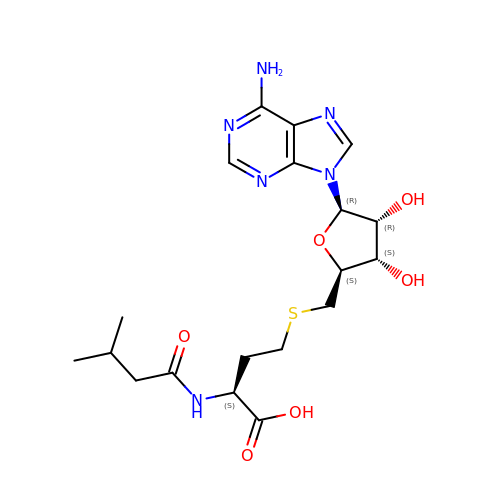(2S)-4-({[(2S,3S,4R,5R)-5-(6-amino-9H-purin-9-yl)-3,4-dihydroxytetrahydrofuran-2-yl]methyl}sulfanyl)-2-[(3-methylbutanoyl)amino]butanoic acid | C19 H28 N6 O6 S | DHVHVJZUMVOUEH-MBRXSIFGSA-N> RSYPAIPRIYAETTLNMLLKRAKKPRVHSIDEYLKDGGYQALEKALNMSPEEIIDWVDKSTLRGRGGAGFPTGKKWKFAVQNPGPRYFICNADEMEPGTFKDRIIIERDPHLLIEGIIISSYAIGANEAYIYIRGEYPAGYYILRDAIEEAKKKGF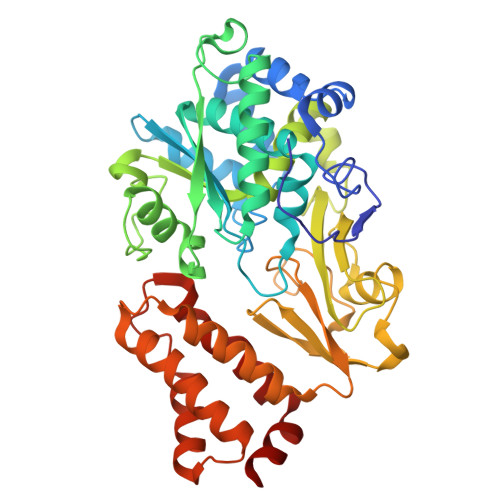LGKNILGSGFDLEIYVARGAGAYICGEETALIESLEGKRGHPRLKPPYPVQKGLWGKPTVVNNVETIANVPFIISMGWEEYRYIGPSDYAGPKLFPVSGKVKKPGVYELPMNTTLREVIFKYAGGTLGNKKVKAVFSGALDCFSSEELDIPMDYSPLGFGGTGTVIVLTEEDDIVEAALKIAEFYEHETCGQCTPCRVGCYEQANLLEKIYKGEATEQDWEGFDFVNRNIQPTSICGLGAVAGRLIRQTLEKFPEEWEKYRK> MRPSAPAISRQTLLDEPRPGSLTIGYEPSEEAQPTENPPRFSWLPDIDDGARYVLRISTDPGFTDKK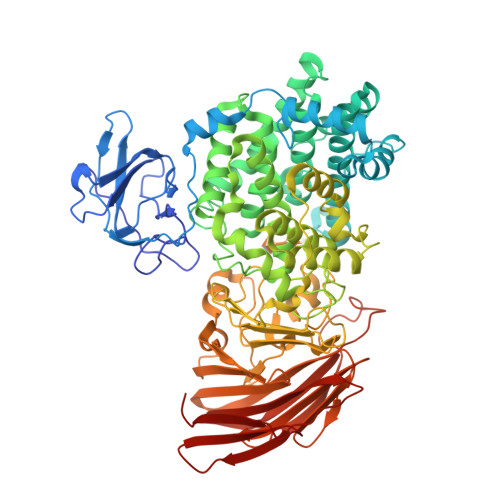TLVFEDLAWNFFTPDEALPDGHYHWCYALWDQKSATAHSNWSTVRSFEISEALPKTPLPGRSARHAAAQTSHPRLWLNSEQLSAFADAVAKDPNHCGWAEFYEKSVEPWLERPVMPEPQPYPNNTRVATLWRQMYIDCQEVIYAIRHLAIAGRVLGRDDLLDASRKWLLAVAAWDTKGATSRAYNDEAGFRVVVALAWGYDWLYDHLSEDERRTVRSVLLERTREVADHVIAHARIHVFPYDSHAVRSLSAVLTPACIALQGESDEAGEWLDYTVEFLATLYSPWAGTDGGWAEGPHYWMTGMAYLIEAANLIRSYIGYDLYQRPFFQNTGRFPLYTKAPGTRRANFGDDSTLGDLPGLKLGYNVRQFAGVTGNGHYQWYFDHIKADATGTEMAFYNYGWWDLNFDDLVYRHDYPQVEAVSPADLPALAVFDDIGWATIQKDMEDPDRHLQFVFKSSPYGSLSASHGDQNAFVLYAHGEDLAIQSGYYVAFNSQMHLNWRRQTRSKNAVLIGGKGQYAEKDKALARRAAGRIVSVEEQPGHVRIVGDATAAYQVANPLVQKVLRETHFVNDSYFVIVDEVECSEPQELQWLCHTLGAPQTGRSSFRYNGRKAGFYGQFVYSSGGTPQISAVEGFPDIDPKEFEGLDIHHHVCATVPAATRHRLVTLLVPYSLKEPKRIFSFIDDQGFSTDIYFSDVDDERFKLSLPKQF> AAPTEAEIIASGKGKFAWPLRGDIISSFGVKGTGQRNDGLNIRAPQGTPVLSSADGEIAYAGNQVPTFGNLVLVKHADGWVTAYAHLSSTNVKMR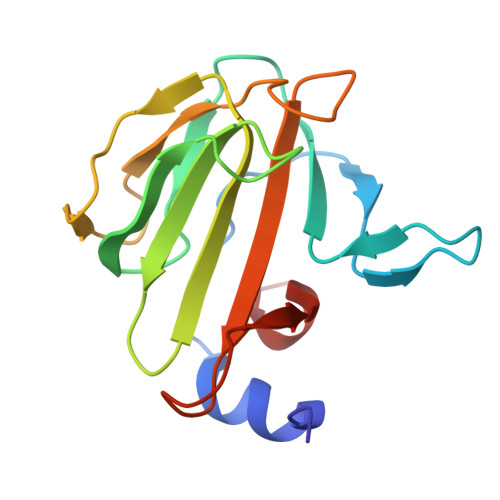QQVKQGEQLGTVGATGGVNEPQLHFEMRYAPTVKDKAKPVDPALVLPR Here, we demonstrate that the centriolar protein SAS-6 forms rod-shaped homodimers that interact through their N-terminal domains to form oligomers. Proteins of the SAS-6 family comprise an N-terminal domain with the evolutionarily conserved PISA motif, followed by a segment with a predicted coiled coil and a less-conserved C-terminal region predicted to be disordered. Furthermore and in conclusion, because these residues are well conserved among SAS-6 orthologs, we propose that the self-assembly of SAS-6 homodimers into a 9-fold symmetric ring structure is a fundamental property at the root of the universal 9-fold symmetry of centrioles.

Next, we determined the structure of the N-terminal globular domain of C. elegans SAS-6 (ceN) by X-ray crystallography. We obtained crystals of a ceN variant and solved its structure to 2.1 Å resolution. The asymmetric unit of the crystal contained a dimer of ceN monomers with local 2-fold symmetry (ceN-dimer). The fold of ceN is reminiscent of that of the XRCC4 family of DNA repair proteins (Junop et al., 2000). We noted that a striking interaction interface in the ceN-dimer was mediated by I154 at the tip of the β6-β7 loop of one monomer, which was inserted deeply into a hydrophobic cavity of the second monomer. Both I154 and the residues shaping the hydrophobic cavity are well conserved among SAS-6 orthologs, suggesting functional relevance. Isothermal titration calorimetry (ITC) experiments yielded a Kd for the N-N interaction of ∼110 ± 30 μM, two orders of magnitude higher than that of the ceCC coiled coil. To address whether I154 mediates ceN-dimer formation, we substituted this residue for the charged residue glutamate (ceN[I154E]). Although the conformation of the domain was not altered by this mutation, AUC experiments revealed that this change abrogated dimer formation. Interestingly, inspection of the ceN-dimer structure suggested that the β6-β7 loop encompassing I154 might promote an interaction between SAS-6 homodimers, as this residue is located diametrically across the ceN domain's C terminus, which proceeds into the coiled coil.

>GSMTSKIALFDQTLIASLLQPLSLNQPDFKAYKTKVKLKISEQRNETSGEKELKFEISRSDDFEFLFSETLNNEKYQILARDHDLTVDFDAFPKVIIQHLLCKNIVKNLEEDGEVDARKKAGYHEIADPGKPTEINIILDAEKNFCSFELFSKTPISKGKIFSIKLHAVR[2x]Zearalenone (ZEN) is a mycoestrogenic polyketide produced by Fusarium graminearum and other phytopathogenic members of the genus Fusarium. ZenA cleaves zearalenone [ZEN, (S,E)-14,16-dihydroxy-3-methyl-3,4,5,6,9,10-hexahydro-1H-benzo[c][1]oxacyclotetradecine-1,7(8H)-dione] to hydrolyzed zearalenone [HZEN, (S,E)-2,4-dihydroxy-6-(10-hydroxy-6-oxoundec-1-en-1-yl)benzoic acid], which decarboxylates spontaneously to decarboxylated hydrolyzed zearalenone [DHZEN, (S,E)-1-(3,5-dihydroxyphenyl)-10-hydroxyundec-1-en-6-one]. Furthermore, we report site-directed mutagenesis as well as structural analysis of the dimeric ZenARe of R. erythropolis and the more thermostable, tetrameric ZenAScfl of Streptomyces coelicoflavus with and without bound ligands. The X-ray crystal structures not only revealed canonical features of α/β hydrolases with a cap domain including a Ser-His-Asp catalytic triad but also unusual features including an uncommon oxyanion hole motif and a peripheral, short antiparallel β-sheet involved in tetramer interactions.

Of the site-directed mutants with a disrupted catalytic triad, ZenAScfl H286Y was used for the structural investigation of enzyme–substrate interactions. The resolutions for ligand bound and unbound structures were 1.53 and 1.92 Å, respectively. For ZenAScfl H286Y cocrystallized with ZEN, refinement was initially carried out with substrate ZEN modeled in the active site. However, the difference density map and a subsequently calculated Polder map revealed a better fit of product HZEN in the active site. The β-resorcylic acid moiety of HZEN was found in a well-defined position at the active site, while the open-chain hydroxyketone moiety appeared flexible. The aromatic side chain of Tyr-286 was positioned as in ZenAScfl H286Y without ligand, but OG of Ser-112 was rotated to occupy the created vacancy. The distance between the atoms that would be forming a covalent bond as a reaction intermediate in wild-type ZenAScfl, carboxylate C12 of HZEN, and OG of Ser-112, is 3.8 Å. However, this distance is only 2.1 Å when measured from the OG of naturally positioned Ser-112 of aligned wild-type ZenAScfl, which therefore appears reaction-competent. The side-chain amide group of Gln-47 as well as OG of Ser-113 form hydrogen bonds with the hydroxyl moiety bound to C2 of HZEN (2.8 and 3.2 Å, respectively). Nonpolar interactions with HZEN are formed by the residues Pro-139, Val-160, Phe-161, and Phe-164.

>[4x]MVTSPALRDVHVPHAYPEQQVDLGEITMNYAEAGDPDRPAVLLIPEQTGSWWSYEEAMGLLSEHFHVYAVDLRGQGRSSWTPKRYSLDNFGNDLVRFIALVVKRPVVVAGNSSGGVLAAWLSAYSMPGQLRGVLCEDPPFFASELVPAHGHSVRQGAGPVFELFRTYLGDQWSVGDWEGFCRAAGASASPMARSFVADGIPQHLQEYDPEWARVFYEGTVGLSCPHERMLGQVKTPVLLTHHMRGIDPETGNLLGALSDEQALRARRLMDSAGVTVDYESVPDASYMMHQSAPARYVEIFTRWAAALAPHHHHHH>[2x]MASYPCHQHASAFDQAARSRGHNNRRTALRPRRQQEATEVRPEQKMPTLLRVYIDGPHGMGKTTTTQLLVALGSRDDIVYVPEPMTYWRVLGA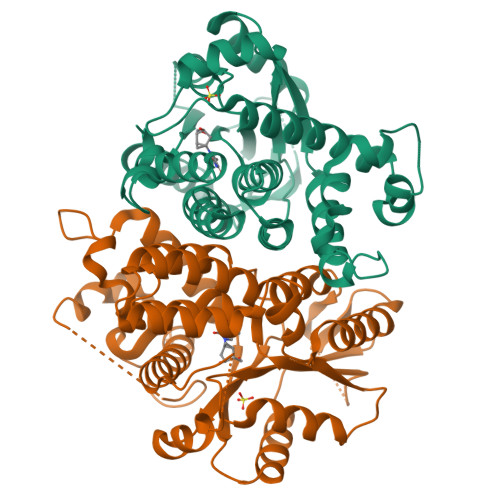SETIANIYTTQHRLDQGEISAGDAAVVMTSAQITMGMPYAVTDAVLAPHIGGEAGSSHAPPPALTLIFDRHPIAALLCYPAARYLMGSMTPQAVLAFVALIPPTLPGTNIVLGALPEDRHIDRLAKRQRPGERLDLAMLAAIRRVYGLLANTVRYLQCGGSWREDWGQLSGTAVPPQGAEPQSNAGPRPHIGDTLFTLFRAPELLAPNGDLYNVFAWALDVLAKRLRSMHVFILDYDQSPAGCRDALLQLTSGMVQTHVTTPGSIPTICDLARTFAREMGEAN> MHHHHHHHHHHLEVLFQGPSYFIFVLGTAGSGKTTLVKALQDYLLNNELDTAIINLDPAVEVLPYKPDIDAREYVDVYDVMNKYELGPNSSLVISVDLLLTKAKELKEDLNQLQANYVLVDTPGQIELFAYRDTGKILSSFISEGSKSVSVFLFDSYLSKDPKSFLSLFLLSSSIKFRIDMPQISVLSKVDLLSSSELERMRSWIEDGSIIDELGSIDEYSFELVKTIVENLESFPIPVSSTNFSGLDQLYAEVQKVLAGGEDFETEEPNPRLA

In the archaeon Sulfolobus acidocaldarius, the GTPase Saci1281 (from hereon: SaGPN) represents the solitary GPN-loop GTPase. Structural analysis of the GTP- and GDP-bound states of the Sulfolobus acidocaldarius GPN enzyme (SaGPN) showed that this central GPN-loop GTPase adopts two distinct quaternary structures. The general structure of SaGPN involves 12 α-helices and a five-stranded, parallel β-sheet that is sandwiched by α6/α8 and α1/α12, respectively. The dimer interface emerges alongside the surface of helices α3, α5, α8, and α11, whereby α8 contributes substantially to the dimeric assembly due to its central position allowing the formation of a hydrophobic pocket.

In the GTP-bound form, the γ-phosphate induces a closed dimeric arrangement by interacting with the GPN region that is relaxed upon hydrolysis to GDP. The eponymous GPN motif (residues G68-N70) is found at the base of α3 (residues N70-L81), which is involved in activation of the inline attacking water molecule (N70) and nucleotide coordination at the substrate pocket of the second protomer. Notably, the water that is suitably positioned for inline attack has still a distance of 3.4 Å from the γ-phosphate of the GppNHp substrate mimic. Accordingly, additional conformational changes for the GPN motif may be feasible during hydrolysis of GTP itself. Additionally, the Walker A motif (GxxxxGK[T/S], x = any amino acid) takes part in nucleotide binding, whereas K14 is responsible for the coordination and orientation of the β/γ phosphates of the nucleotide; T15 is the only proteinaceous part of the octahedral Mg2+ coordination sphere. Mg2+ coordination is also supported by the Walker B motif (hhhhD/E, h = hydrophobic), which interacts indirectly with the Mg2+ ion over a water bridge to D102; the latter residue also forms a hydrogen bond with the hydroxyl moiety of T15. As a consequence, a water molecule that is coordinated between D38 from the G2 motif and N70′ of the GPN motif is now found in an inline attack position for initiating the SN2 reaction at the γ-phosphate. When deprotonated, D38 acts here as a general base for transient formation of the attacking hydroxide nucleophile like the corresponding residue in the G2 box of other SIMIBI GTPases. Overall, the GTP-bound state of GPN-loop GTPases with its closed GPN-lid corresponds to a ‘locked’ state. In addition to helices α3 and α4 incorporating more deuterium similar to the GDP-bound state, the roof-constituting helices α9-α11 (residues E178-N212) specifically for GppNHp/SaGPN incorporate more deuterium (peptides L151-L168, R183-L195, and K207-L213).>MALNSINTNAGAMIALQNLNGTNSELTTVQQRINTGKKIASAKDN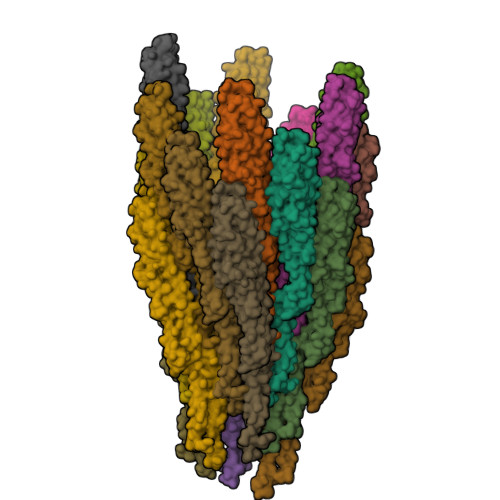GAIWATAKNQSATAASMNAVKDSLQRGQSTIDVALAAGDTITDLLGKMKEKALAASDTSLNTASFNALKSDFDSLRDQIEKAATNAKFNGVSIADGSTTKLTFLANSDGSGFTVNAKTISLAGIGLTTTSTFTTAAAAKTMIGTIDTALQTATNKLASLGTSSVGLDTHLTFVGKLQDSLDAGVGNLVDADLAKESAKLQSLQTKQQLGVQALSIANQSSSSILSLFR[20x]> LLVVGPKFIRANQEYTLVISNFNSQLSKVDLLLKLEGETDNGLSVLNVTKMVDVRRNMNRMINFNMPEDLTAGNYKITIDGQRGFSFHKEAELVYLSKSISGLIQVDKPVFKPGDTVNFRVIVLDTELKPPARVKSVYVTIRDPQRNVIRKWSTAKLYAGVFESDLQIAPTPMLGVWNISVEVEGEELVSKTFEVKEYVLSTFDVQVMPSVIPLEEHQAVNLTIEANYHFGKPVQGVAKVELYLDDDKLKLKKELTVYGKGQVELRFDNFAMDADQQDVPVKVSFVEQYTNRTVVKQSQITVYRYAYRVELIKESPQFRPGLPFKCALQFTHHDGTPAKGISGKVEVSDVRFETTTTSDNDGLIKLELQPSEGTEQLSIHFNAVDGFFFYEDVNKVETVTDAYIKLELKSPIKRNKLMRFMVTCTERMTFFVYYVMSKGNIIDAGFMRPNKQPKYLLQLNATEKMIPRAKILIATVAGRTVVYDFADLAFQELRNNFDLSIDEQEIKPGRQIELSMSGRPGAYVGLAAYDKALLLFNKNHDLFWEDIGQVFDGFHAINENEFDIFHSLGLFARTLDDILFDSANEKTGRNALQSGKPIGKLVSYRTNFQESWLWKNVSIGRSGSRKLIEVVPDTTTSWYLTGFSIDPVYGLGIIKKPIQFTTVQPFYIVENLPYSIKRGEAVVLQFTLFNNLGAEYIADVTLYNVANQTEFVGRPNTDLSYTKSVSVPPKVGVPISFLIKARKLGEMAVRVKASIMLGHETDALEKVIRVMPESLVQPRMDTRFFCFDDHKNQTFPINLDINKKADSGSTKIEFRLNPNLLTTVIKNLDHLLGVPTGCGEQNMVKFVPNILVLDYLHAIGSKEQHLIDKATNLLRQGYQNQMRYRQTDGSFGLWETTNGSVFLTAFVGTSMQTAVKYISDIDAAMVEKALDWLASKQHFSGRFDKAGAEYHKEMQGGLRNGVALTSYVLMALLENDIAKAKHAEVIQKGMTYLSNQFGSINNA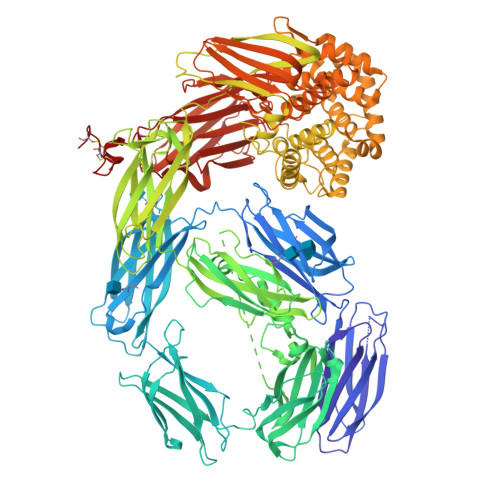YDLSIATYAMMLNGHTMKEEALNKLIDMSFIDADKNERFWNTTNPIETTAYALLSFVMAEKYTDGIPVMNWLVNQRYVTGSFPSTQDTFVGLKALTKMAEKISPSRNDYTVQLKYKKSAKYFKINSEQIDVENFVDIPEDTKKLEINVGGIGFGLLEVVYQFNLNLVNFENRFQLDLEKQNTGSDYELRLKVCASYIPQLTDRRSNMALIEVTLPSGYVVDRNPISEQTKVNPIQKTEIRYGGTSVVLYYDNMGSERNCFTLTAYRRFKVALKRPAYVVVYDYYNTNLNAIKVYEVDKQNLCEICDEEDCPAECGGHHHHHH> DDDLVDAEGNLVENGGTYYLLPHIWAHGGGIETAKTGNEPCPLTVVRSPNEVSKGEPIRISSQFRSLFIPRGSLVALGFANPPSCAASPWWTVVDSPQGPAVKLSQQKLPEKDI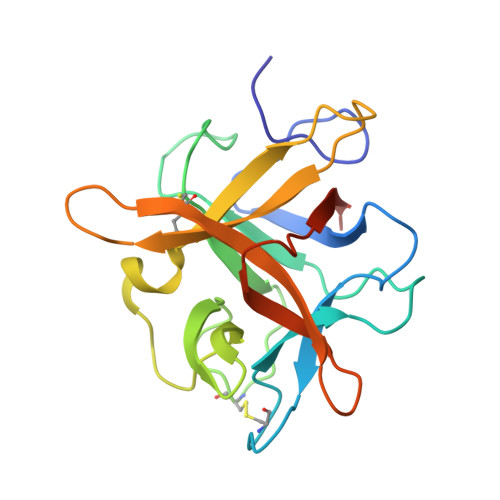LVFKFEKVSHSNIHVYKLLYCQHDEEDVKCDQYIGIHRDRNGNRRLVVTEENPLELVLLKAKSETASSH>[2x]MFEQRVNSDVLTVSTVNSQDQVTQKPLRDSVKQA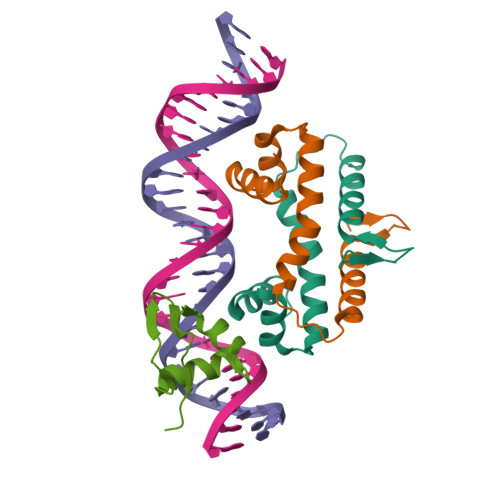LKNYFAQLNGQDVNDLYELVLAEVEQPLLDMVMQYTRGNQTRAALMMGINRGTLRKKLKKYGMN;> MYLTLQEWNARQRRPRSLETVRRWVRESRIFPPPVKDGREYLFHESAVKVDLNRP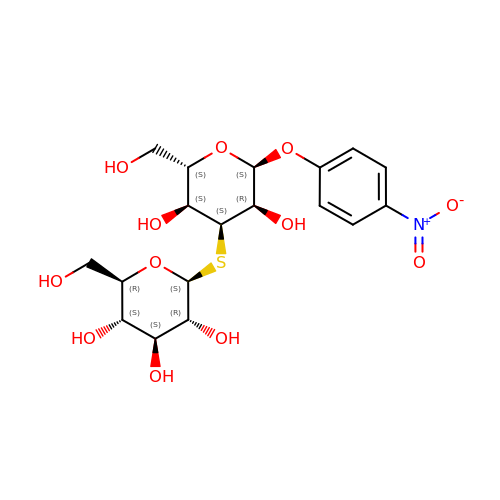(2~{R},3~{S},4~{S},5~{R},6~{S})-2-(hydroxymethyl)-6-[(2~{S},3~{S},4~{S},5~{R},6~{S})-2-(hydroxymethyl)-6-(4-nitrophenoxy)-3,5-bis(oxidanyl)oxan-4-yl]sulfanyl-oxane-3,4,5-triol | C18 H25 N O12 S | JHLJVHIWBCGKQZ-KZPLUMROSA-N> MAVLKIISWNVNGLRAVHRKGFLKWFMEEKPDILCLQEIKAAPEQLPRKLRHVEGYRSFFTPAERKGYSGVAMYTKVPPSSLREGFGVERFDTEGRIQIADFDDFLLYNIYFPNGAMSEERLKYKLEFYDAFLEDVNRERDSGRNV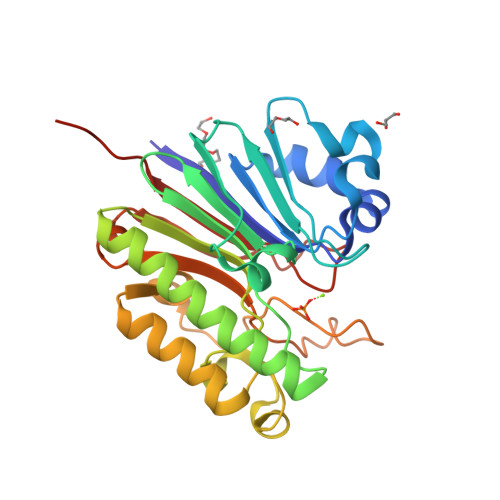IICGDFNTAHREIDLARPKENSNVSGFLPVERAWIDKFIENGYVDTFRMFNSDPGQYTWWSYRTRARERNVGWRLDYFFVNEEFKGKVKRSWILSDVMGSDHCPIGLEIELLEHHHHHH> SHAKDVKI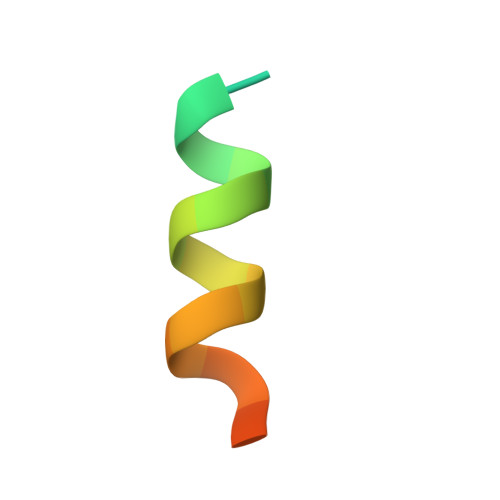QETIRKLNRFKPT> SITGISPITEYLA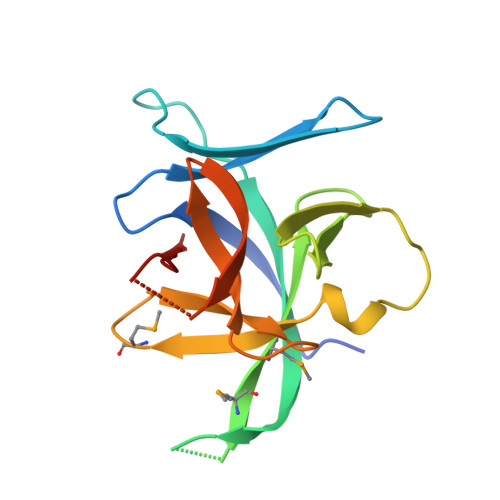SLSTYNDQSITFALEDESYEIYVEDLKKDEKKDKVLLSYYESQHPSNESGDGVDGKMLMVTLSPTKDFWLHANNKEHSVELHKCEKPLPDQAFFVLHNMHSNCVSFECKTDPGVFIGVKDNHLALIKVDSSENLCTENILFKLSET>GAMGSEISKTEAGQYSVSAPEHKGLVLSGGGAKGISYLGMIQALQERGKIKNLTHVSGASAGAMTASILAVGMDIKDIKKLIEGLDITKLLDNSGVGFRARGDRFRNILDVIYMMQMKKHLESVQQPIPPEQQMNYGILKQKIALYEDKLSRAGIVINNVDDIINLTKSVKDLEKLDKALNSIPTELKGAKGEQLENPRLTLGDLGRLRELLPEENKHLIKNLSVVVTNQTKHELERYSEDTTPQQSIAQVVQWSGAHPVLFVPGRNAKGEYIADGGILDNMPEIEGLDREEVLCVKAEAGTAFEDRVNKAKQSAMEAISWFKARMDSLVEATIGGKWLHATSSVLNREKVYYNIDNMIYINTGEVTTTNTSPTPEQRARAVKNGYDQTMQLLDSHKQTFDHPLMAILYIGHDKLKDALIDEKSEKEIFEASAHAQAILHLQEQIVKEMNDGDYSSVQNYLDQIEDILTVDAKMDDIQKEKAFALCIKQVNFLSEGKLETYLNKVEAEAKAAAEPSWATKILNLLWAPIEWVVSLFKGPAQDFKVEVQPEP[4x];>[4x]GAMGSKICQFKLVLLGESAVGKSSLVLRFVKGQFHEYQESTIGAAFLTQTVCLDDTTVKFEIWDTAGLERYH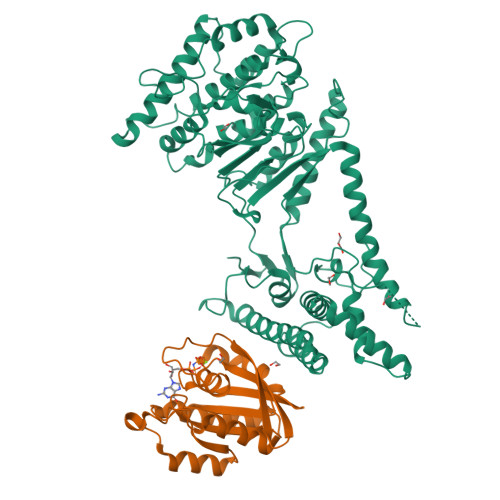SLAPMYYRGAQAAIVVYDITNTDTFARAKNWVKELQRQASPNIVIALAGNKADLASKRAVEFQEAQAYADDNSLLFMETSAKTAMNVNEIFMAIAKKL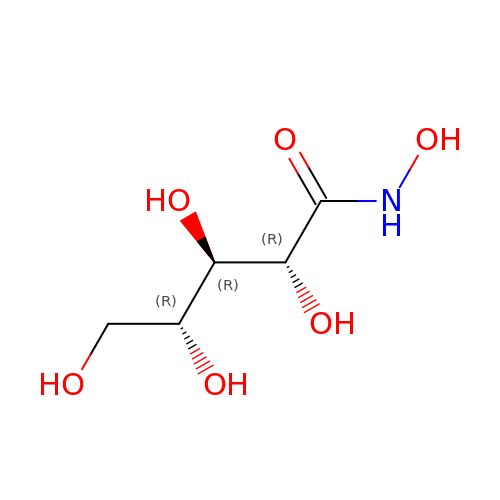(2R,3R,4R)-N,2,3,4,5-pentakis(oxidanyl)pentanamide | C5 H11 N O6 | AGVYHANDLPZRFS-BXXZVTAOSA-N> MVGGV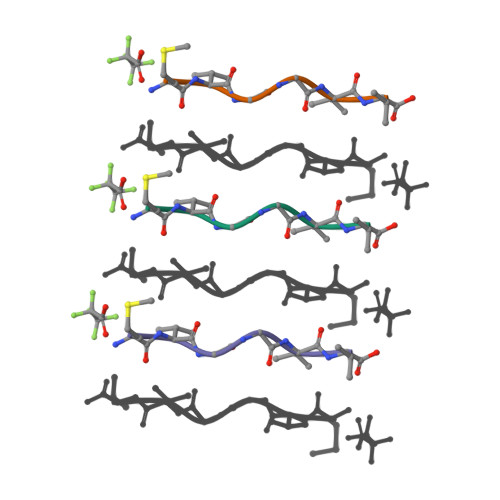V methyl 6-O-(heptylcarbamoyl)-beta-L-altropyranoside 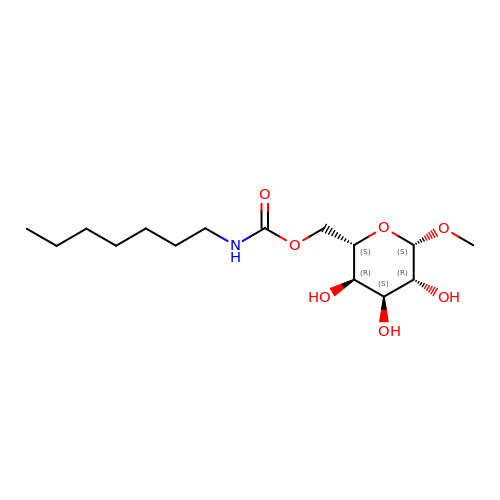| C15 H29 N O7 | XPIVOYOQXKNYHA-YHQUGGNUSA-N>MHHHHHHAAGIPMNNPAIKRIGNHITKSPEDKREYRGLELANGIKVLLISDPTTDKSSAALDVHIGSLSDPPNIAGLSHFCEHMLFLGTKKYPKENEYSQFLSEHAGSSNAFTSGEHTNYYFDVSHEHLEGALDRFAQFFLCPLFDESCKDREVNAVDSEHEKNVMNDAWRLFQLEKATGNPKHPFSKFGTGNKYTLETRPNQEGIDVRQELLKFHSAYYSSNLMAVCVLGRESLDDLTNLVVKLFSEVENKNVPLPEFPEHPFQEEHLKQLYKIVPIKDIRNLYVTFPIPDLQKYYKSNPGHYLGHLIGHEGPGSLLSELKSKGWVNTLVGGQKEGARGFMFFIINVDLTEEGLLHVEDIILHMFQYIQKLRAEGPQEWVFQECKDLNAVAFRFKDKERPRGYTSKIAGILHYYPLEEVLTAEYLLEEFRPDLIEMVLDKLRPENVRVAIVSKSFEGKTDRTEEWYGTQYKQEAIPDEVIKKWQNADLNGKFKLPTKNEFIPTNFEILPLEKEATPYPALIKDTAMSKLWFKQDDKFFLPKACLNFEFFSPFAYVDPLHCNMAYLYLELLKDS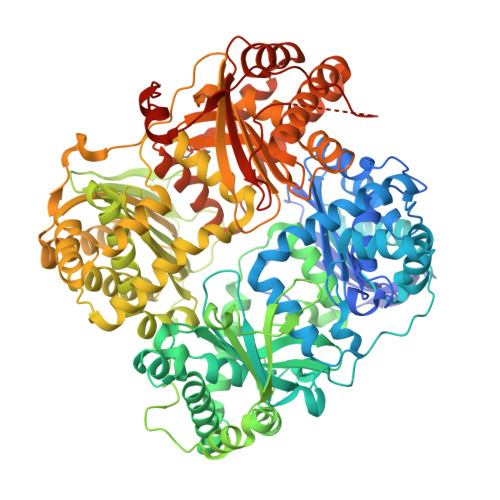LNEYAYAAELAGLSYDLQNTIYGMYLSVKGYNDKQPILLKKIIEKMATFEIDEKRFEIIKEAYMRSLNNFRAEQPHQHAMYYLRLLMTEVAWTKDELKEALDDVTLPRLKAFIPQLLSRLHIEALLHGNITKQAALGIMQMVEDTLIEHAHTKPLLPSQLVRYREVQLPDRGWFVYQQRNEVHNNCGIEIYYQTDMQSTSENMFLELFCQIISEPCFNTLRTKEQLGFIVFSGPRRANGIQGLRFIIQSEKPPHYLESRVEAFLITMEKSIEDMTEEAFQKHIQALAIRRLDKPKKLSAECAKYWGEIISQQYNFDRDNTEVAYLKTLTKEDIIKFYKEMLAVDAPRRHKVSVHVLAREMDSCPVVGEFPCQNDINLSQAPALPQPEVIQNMTEFKRGLPLFPLVKPHINFMAAKL[2x]> SEIPLPIPVKVI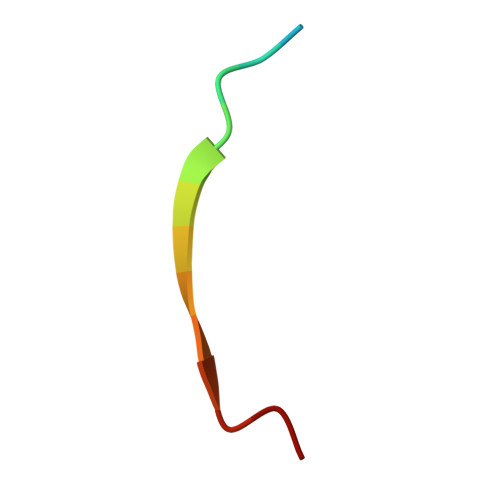NTL>DLLVPKLTASVTDGAVGVTVDAPVSVTAADGVLAAVTMVNENGRPVAGRLSPDGLRWSTTEQLGYNRRYTLNATALGLGGAATRQLTFQTSSPAHLTMPYVMPGDGEVVGVGEPVAIRFDENIADRGAAEKAIKITTNPPVEGAFYWLNNREVR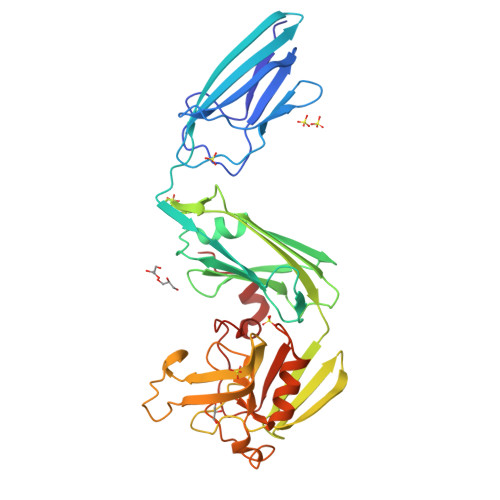WRPEHFWKPGTAVDVAVNTYGVDLGEGMFGEDNVQTHFTIGDEVIATADDNTKILTVRVNGEVVKSMPTSMGKDSTPTANGIYIVGSRYKHIIMDSSTYGVPVNSPNGYRTDVDWATQISYSGVFVHSAPWSVGAQGHTNTSHGCLNVSPSNAQWFYDHVKRGDIVEVVNTVGGTLPGIDGLGDWNIPWDQWRAGNAK[2x]>HMINKKSLLQNLLSKCKTTFQQSFTNANITLKDEKWLKNVRTAYFVCDHDGSVELAYLPNVLPKELVEEFTEKFESIQTGRKKDTGYSGILDNSMPFNYVTADLSQELGQYLSEIVNPQINYYISKLLTCVSSRTINYLVSLNDSYYALNNCLYPSTAFNSLKPSNDGHRIRKPHKDNLDITPSSLFYFGNFQNTEGYLELTDKNCKVFVQPGDVLFFKGNEYKHVVANITSGWRIGLV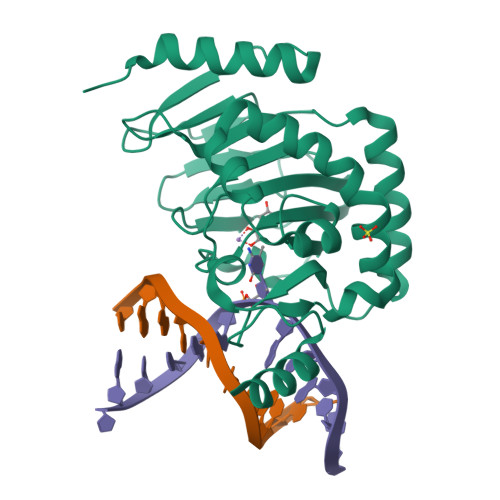YFAHKGSKTKPYYEDTQKNSLKIHKETK[2x]> HHMGTNGTMMQYFEWHLPNDGQHWNRLRDDASNLRNRGITAIWIPPAWKGTSQNDVGYGAYDLYDLGEFNQKGTVRTKYGTRSQLESAIHALKNNGVQVYGDVVMNHKGGADATENVLAVEVNPNNRNQEISGDYTIEAWTKFDFPGRGNTYSDFKWRWYHFDGVDWDQSRQFQNRIYKFRGDGKAWDWEVDSENGNYDYLMYADVDMDHPEVVNELRRWGEWYTNTLNLDGFRIDAVKHIKYSFTRDWLTHVRNATGKEMFAVAEFWKNDLGALENYLNKTNWNHSVFDVPLHYNLYNASNSGGNYDMAKLLNGTVVQKHPMHAVTFVDNHDSQPGESLESFVQEWFKPLAYALILTREQGYPSVFYGDYYGIPTHSV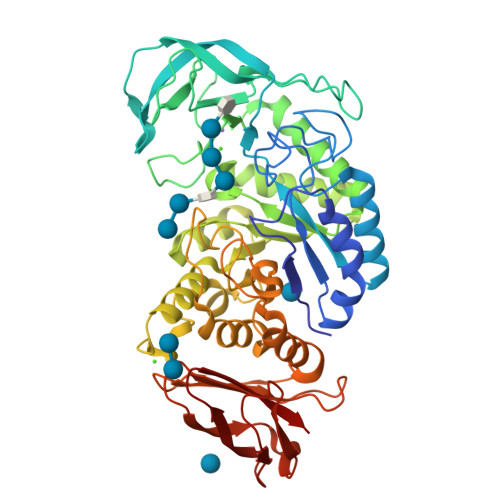PAMKAKIDPILEARQNFAYGTQHDYFDHHNIIGWTREGNTTHPNSGLATIMSDGPGGEKWMYVGQNKAGQVWHDITGNKPGTVTINADGWANFSVNGGSVSIWVKR> MPFVNKQFNYKDPVNGVDIAYIKIPNAGQMQPVKAFKIHNKIWVIPERDTFTNPEEGDLNPPPEAKQVPVSYYDSTYLSTDNEKDNYLKGVTKLFERIYSTDLGRMLLTSIVRGIPFWGGSTIDTELKVIDTNCINVIQPDGSYRSEELNLVIIGPSADIIQFECKSFGHEVLNLTRNGYGSTQ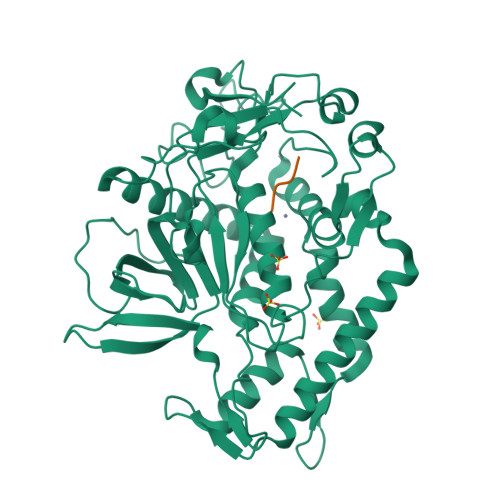YIRFSPDFTFGFEESLEVDTNPLLGAGKFATDPAVTLAHELIHAGHRLYGIAINPNRVFKVNTNAYYEMSGLEVSFEELRTFGGHDAKFIDSLQENEFRLYYYNKFKDIASTLNKAKSIVGTTASLQYMKNVFKEKYLLSEDTSGKFSVDKLKFDKLYKMLTEIYTEDNFVKFFKVLNRKTYLNFDKAVFKINIVPKVNYTIYDGFNLRNTNLAANFNGQNTEINNMNFTKLKNFTGLFELEHHHHHH;> RRGMX> GMTSNGQQGKPNLPEKDNLPRELGTQRINSPIARMGMFGAKTTGDTSGYGRLRVYRHVPAAAQRPYSDPSDPRTAYFDEVADALERSLKEIGTPYDTAISRVVVDRGEITFHVQREHLLDVATRL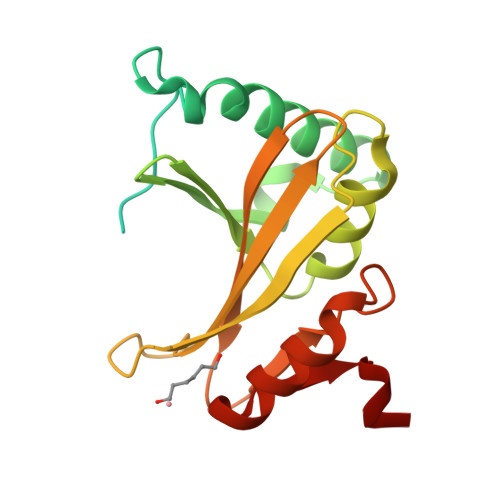RDDPALRFELCLGVTGVHYPEDEGNELHAVYALRSITHNYEIRLEVSCPDSDPHIPSIVSVYPTNDWHEREAWDFFGIIFDGHPALTR> MSLKYKLIVLDLDGTLTNSKKEISSRNRETLIRIQEQGIRLVL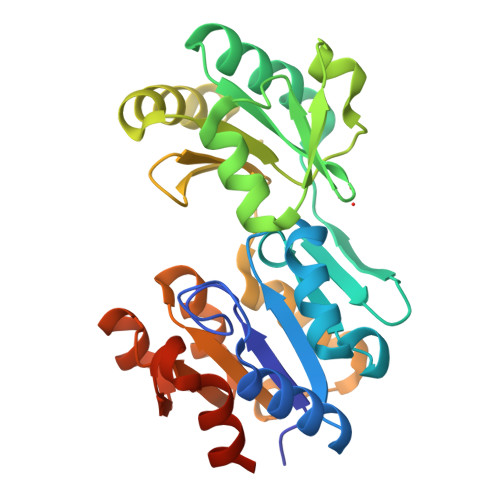ASGRPTYGIVPLANELRMNEFGGFILSYNGGEIINWESKEMMYENVLPNEVVPVLYECARTNHLSILTYDGAEIVTENSLDPYVQKEAFLNKMAIRETNDFLTDITLPVAKCLIVGDAGKLIPVESELCIRLQGKINVFRSEPYFLELVPQGIDKALSLSVLLENIGMTREEVIAIGDGYNDLSMIKFAGMGVAMGNAQEPVKKAADYITLTNDEDGVAEAIERIFNVEGHHHHHH>[4x]MEEQIVPFYGKHQAGITTAHQTY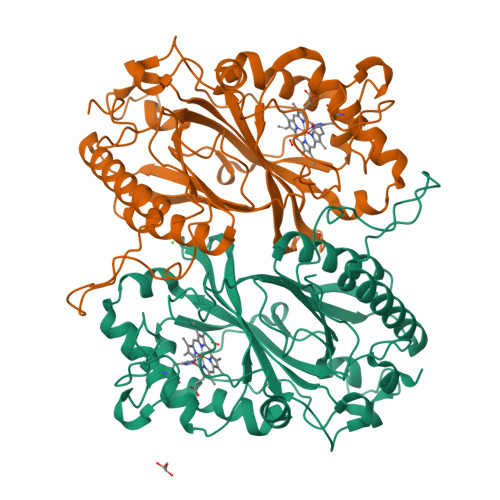VYFAALDVTAKEKSDIITLFRNWTSLTQMLTSGKKMSAEQRNQYLPPQDTGESADLSPSNLTVTFGFGPSFFEKDGKDRFGLKSKKPKHLAALPAMPNDNLDEKQGGGDICIQVCADDEQVAFHALRNLLNQAVGTCEVRFVNKGFLSGGKNGETPRNLFGFKDGTGNQSTEDDSLMNSIVWVQSGEPDWMTGGTYMAFRKIKMFLEIWDRSSLKDQEDTFGRRKSSGAPFGQKKETDPVKLNQIPSNSHVSLAKSTGKQILRRAFSYTEGLDPKTGYMDAGLLFISFQKNPDNQFIPMLKALSAKDALNEYTQTIGSALYACPGGCKKGEYIAQRLLES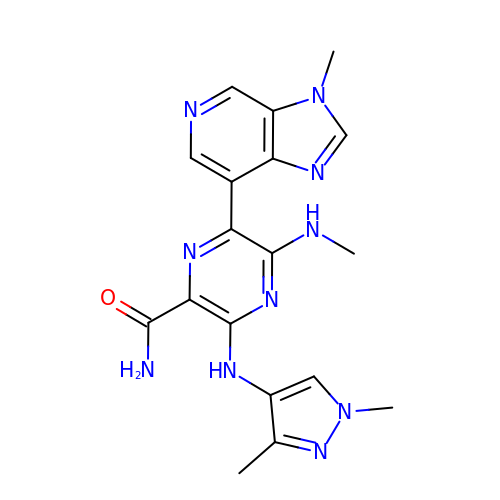3-[(1,3-dimethylpyrazol-4-yl)amino]-5-(methylamino)-6-(3-methylimidazo[4,5-c]pyridin-7-yl)pyrazine-2-carboxamide | C18 H20 N10 O | BUGHKAJGIGJJGX-UHFFFAOYSA-N> MFSQIVLLLSAFIYVASATARRGTIKGRLDLAASNITGFVSTRTSFKLYQIGNFSTEYPYTSTTMFQDDEGNFEFANLPLNDGVNETTYYVMYPASMDFNLKPNRILIEFKNLENGTLQLNAFKNFFGREYFPSKDITYPEKLQSMKVHPYITVELLHKAPIRSYLQARNVSIFSTGIVGNILNS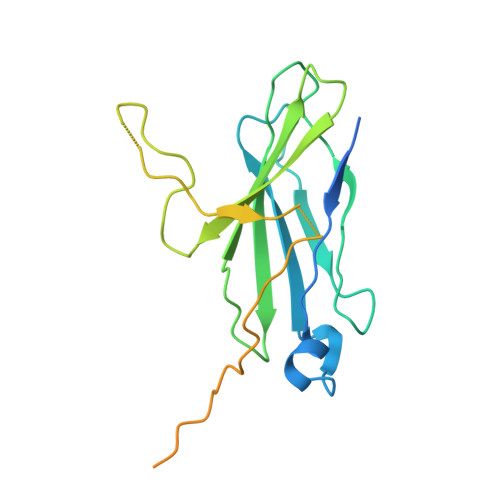RWKLAGVITLIALVVFPIIVEKLDPETARAIREEAKRKQREKYAAVASK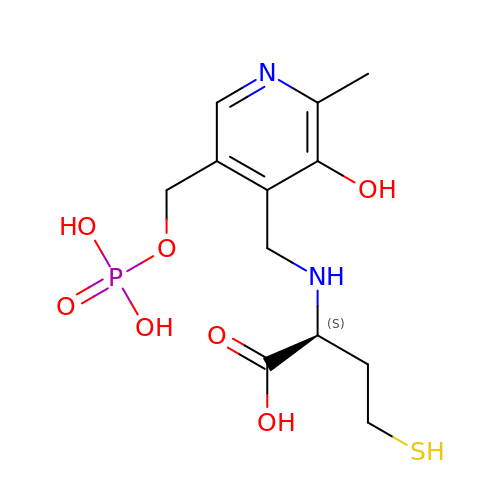(2~{S})-2-[[2-methyl-3-oxidanyl-5-(phosphonooxymethyl)pyridin-4-yl]methylamino]-4-sulfanyl-butanoic acid | C12 H19 N2 O7 P S | PXCMMZUTCUCUSM-JTQLQIEISA-N Our focus here is on a PLP especially identified as being involved in neurodevelopment, astrotacin-2 (ASTN-2). ASTN-1 and ASTN-2 have been shown to interact directly with each other in vitro in a calcium-independent way with multiple regions of each protein apparently contributing to their interface. Both ASTN-1 and ASTN-2 are integral membrane proteins in which a large C-terminal domain (extracellular for ASTN-1, endosome luminal for ASTN-2) is complemented by an N-terminal cytosolic domain suspended between two transmembrane α-helices. Thus, the endosomal regions of ASTN-2 comprise a smaller N-terminal domain and a larger C-terminal domain whose structure we report here and which we refer to as its endodomain. We describe its unique combination of a canonical MACPF/CDC domain with a minimal epidermal growth factor (EGF)-like repeat (EGF-4), a previously unobserved type of fibronectin type III (Fn(III)) domain in which an additional two β-strands are folded across the core, and an annexin-like domain.

The movement of ASTN-2 through the endolysosomal system suggests that its activity might be regulated by pH. We have determined structures of the endodomain at pH 7.5 and pH 5 and of the MACPF/CDC domain alone at pH 4, and find the regions of ASTN-2 resolved to be remarkably insensitive to acidification. In an attempt to investigate the effect of reduced pH on the ASTN-2 structure, we obtained crystals of constructs consisting of EGF-3 to the C-terminus (residues 649–1288) at pH 5 and of EGF-3 plus the MACPF domain at pH 4 (residues 649–984), though in neither case was EGF-3 resolved in the resulting structures. ASTN-2649-1288 was crystallized in 0.1 M MES, pH 5.0–6.0, 5% PEG 6000. The crystal structure of the MACPF domain C-terminus at pH 5 and of the MACPF domain alone at pH 4 were solved by molecular replacement using copy A of the structure solved at pH 7.5 in PHASER and refinement was carried out in PHENIX. The conformations of the lower pH forms of ASTN-2 are very similar to the equivalent regions of the neutral pH structure (RMSDs 0.23 Å (pH 5) and 1.52 Å (pH 4)). Yet overall these regions of ASTN-2 seem remarkably insensitive to pH suggesting that, if pH is a triggering factor in ASTN-2 activity as it moves through the endolysosomal system, the sensor is not in these parts of the structure. The junction between the EGF-4 and Fn(III) domains contains density which is not part of the ASTN-2 polypeptide and which can plausibly be modelled as an inositol triphosphate bound within a surface cavity.

> KFNDTLFGEMLHGYNNRTQHVNQGQVFQMTFRENNFIKDFPQLADGLLVIPLPVEEQCRGVLSEPLPDLQLLTGDIRYDEAMGYPMVQQWRVRSNLYRVKLSTITLAAGFTNVLKILTKESSREELLSFIQHYGSHYIAEALYGSELTCIIHFPSKKVQQQLWLQYQKETTELGSKKELKSMPFITYLSGLLTAQMLSDDQLISGVEIRCEEKGRCPSTCHLCRRPGKEQLSPTPVLLEINRVVPLYTLIQDNGTKEAFKSALMSSYWCSGKGDVIDDWCRCDLSAFDANGLPNCSPLLQPVLRLSPTVEPSSTVVSLEWVDVQPAIGTKVSDYILQHKKVDEYTDTDLYTGEFLSFADDLLSGLGTSCVAAGRSHGEVPEVSIYSVIFKCLEPDGLYKFTLYAVDTRGRHSELSTVTLRTACPLVDDNKAEEIADKIYNLYNGYTSGKEQQMAYNTLMEVSASMLFRVQHHYNSHYEKFGDFVWRSEDELGPRKAHLILRRLERVSSHCSSLLRSAYIQSRVETVPYLFCRSEEVRPAGMVWYSILKDTKITCEEKMVSMARNTYGESKGR> GMSSDVQKGDNLETPGARDLLLQTASNIMREGDVVDISLSELSLRSGLNSALVKYYFGNKAGLLKALLDRDMENIVKSVDALLAKDDMSPEAKLRRHISKCIDTYYDYPYLNRLLMRLVRDSDEAEAKRIADQYLLPLHRAYNRFIGEGVKAGVFRPINPQLFYFTVTGAADRF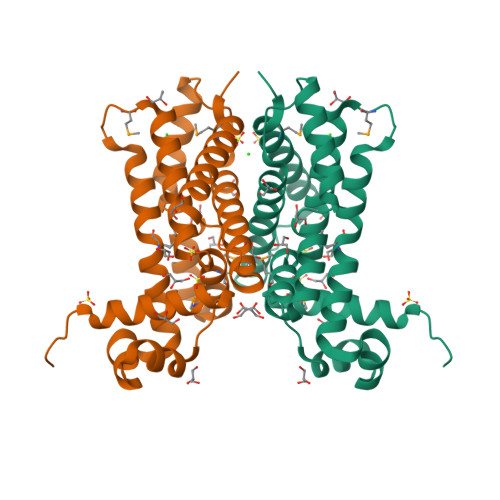FSARLVLKHCFDQDTLTEQLRDSYREHTVDFIMAGILAH>MGPGFDFAQA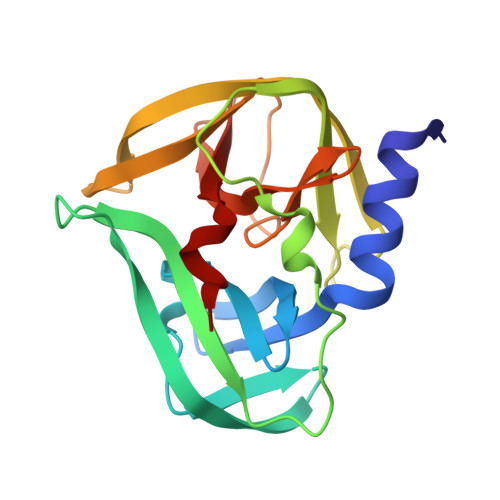IMKKNTVIARTEKGEFTMLGVYDRVAVIPTHASVGEIIYINDVETRVLDACALRDLTDTNLEITIVKLDRNQKFRDIRHFLPRCEDDYNDAVLSVHTSKFPNMYIPVGQVTNYGFLNLGGTPTHRILMYNFPTRAGQCGGVVTTTGKVIGIHVGGNGAQGFAAMLLHSYFTD[2x]> GPLGSMVSGVGGSGGGRGGGRGGEEEPSSSHTPNNRRGGEQAQSSGTKSLRPRSNTESMSKAIQQYTVDARLHAVFEQSGESGKSFDYSQSLKTTTYGSSVPEQQITAYLSRIQRGGYIQPFGCMIAVDESSFRIIGYSENAREMLGIMPQSVPTLEKPEILAMGTDVRSLFTSSSSILLERAFVARE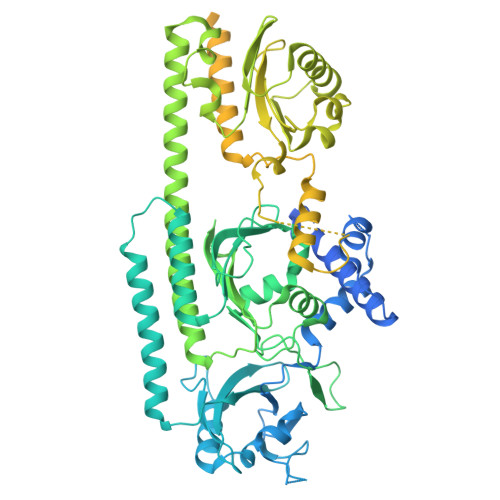ITLLNPVWIHSKNTGKPFYAILHRIDVGVVIDLEPARTEDPALSIAGAVQSQKLAVRAISQLQALPGGDIKLLCDTVVESVRDLTGYDRVMVHKFHEDEHGEVVAESKRDDLEPYIGLHYPATDIPQASRFLFKQNRVRMIVDCNATPVLVVQDDRLTQSMCLVGSTLRAPHGCHSQYMANMGSIASLAMAVIINGNEDDGSNVASGRSSMRLWGLVVCHHTSSRCIPFPLRYACEFLMQAFGLQLNMELQLALQMSEKRVLRTQTLLCDMLLRDSPAGIVTQSPSIMDLVKCDGAAFLYHGKYYPLGVAPSEVQIKDVVEWLLANHADSTGLSTDSLGDAGYPGAAALGDAVCGMAVAYITKRDFLFWFRSHTAKEIKWGGAKHHPEDKDDGQRMHPRSSFQAFLEVVKSRSQPWETAEMDAIHSLQLILRDSFKESEAAMNSKVVDGVVQPCRDMAGEQGIDELGAVAREMVRLIETATVPIFAVDAGGCINGWNAKIAELTGLSVEEAMGKSLVSDLIYKENEATVNKLLSRALRGDEEKNVEVKLKTFSPELQGKAVFVVVNACSSKDYLNNIVGVCFVGQDVTSQKIVMDKFINIQGDYKAIVHSPNPLIPPIFAADENTCCLEWNMAMEKLTGWSRSEVIGKMIVGEVFGSCCMLKGPDALTKFMIVLHNAIGGQDTDKFPFPFFDRNGKFVQALLTANKRVSLEGKVIGAFCFLQIPS UdgX excises uracil from uracil-containing DNA to concurrently form a covalent bond with the resulting AP-DNA. Structurally, UdgX is highly similar to family-4 UDGs (F4-UDGs). However, UdgX is unique in possessing a flexible R-loop (105KRRIH109). Our earlier studies allowed us to propose a reaction mechanism of UdgX, which involves the formation of a covalent bond between H109 of UdgX with the C1′ position of the target deoxyribose sugar concurrently with the uracil excision from this site in DNA.

Substitutions of His109 in MsmUdgX with Ser, Gly, Ala, Gln, Cys and Lys showed the loss of its covalent complex formation with DNA but gained canonical UDG activities. However, H109 substitutions by Gln or Lys, showed poor activity. Both Cys and Ala mutations of H109 showed intermediate Kcat/Km values. However, to better understand the mechanism of uracil excision by the H109 mutants, we determined their structures along with a pentameric DNA, TTUTT by X-ray crystallography. The DNA backbone could not be modelled into the experimental electron density map in any of the mutant structures that were determined. Nonetheless, all structures revealed the excised uracil and the side chain substitutions at position 109. The structures also revealed invariant interactions of N91 and H178 with uracil. When we arranged the mutants in the order of increasing cavity sizes (left), we noted that the canonical UDG activity of the mutants increased with their increasing cavity sizes to begin with and then with a further increase in the cavity size, the UDG activity declined (right). It suggested that the initial increase in UDG activity (H109K to H109Q to H109G) occurred because of the efficiency with which the water molecule could be localized to make a nucleophilic attack on the C1′ position. However, a further increase in the cavity size (H109S to H109C to H109A) perhaps destabilizes the bound water, thereby decreasing the UDG activity.

> AGAQDFVPHTADLAELAAAAGECRGCGLYRDATQAVFGAGGRSARIMMIGEQPGDKEDLAGLPFVGPAGRLLDRALEAADIDRDALYVTNAVKHFKFTRAAGGKRRIAKTPSRTEVVACRPWLIAEMTSVEPDVVVLLGATAAKALLGNDFRVTQHRGEVLHVDDVPGDPALVATVHPSSLLRGPKEERESAFAGLVDDLRVAADV(3~{R})-3-[2-[4-(2-azanylethylamino)cyclohexyl]ethanoylamino]-2-oxidanyl-3,4-dihydro-1,2-benzoxaborinine-8-carboxylic 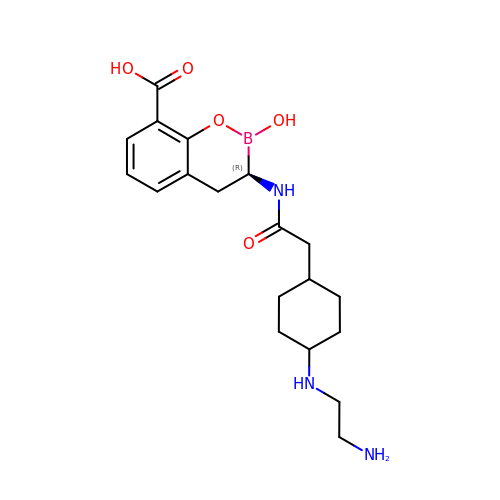acid | C19 H28 B N3 O5 | PFZUWUXKQPRWAL-NOLJZWGESA-N>[4x]MHHHHHHGSMENQVKVLNLW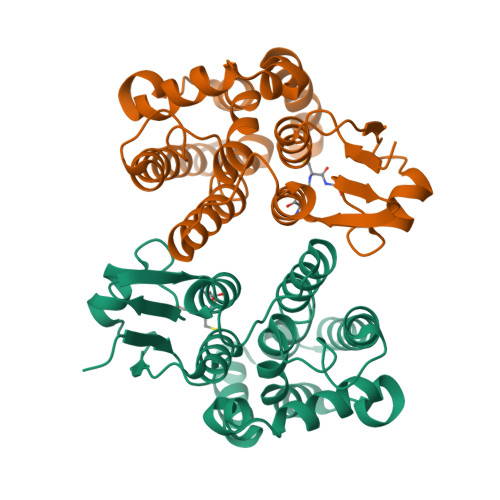ASPFGLRVLVGLEEKGVKYEYQEENLASKSELLLKMNPIHKKIPVLIHNDKPVLESLIIVEYIDEAWPNTNPFMPSSAYERARARFWADFVDKKLYDNGGALIMKCKGEAQEEAKRNMLEYLGLLEGALDELSGGIKPYFGGEKFGYMDIAFIPFASWFQAWEVMGNWKIPLETQFPRLHEWVNACMERESVKKVLPHPEKVAEFAMQMRRRFVGSD> IWIAQ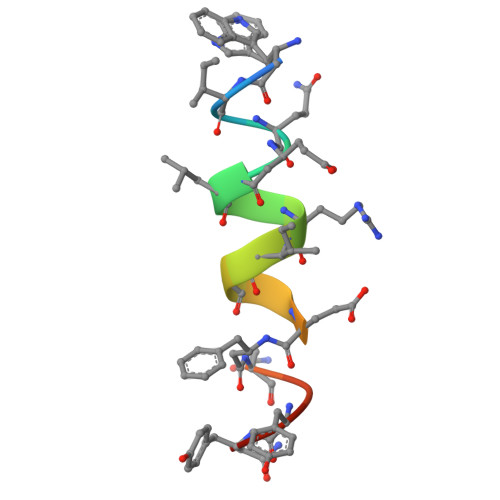ELRRXGDEXNAYYX>[2x]MTTFLIKHKASGKFLHPYGGSSNPANNTKLVLHSDIHERMYFQFDVVDERWGYIKHVASGKIVHP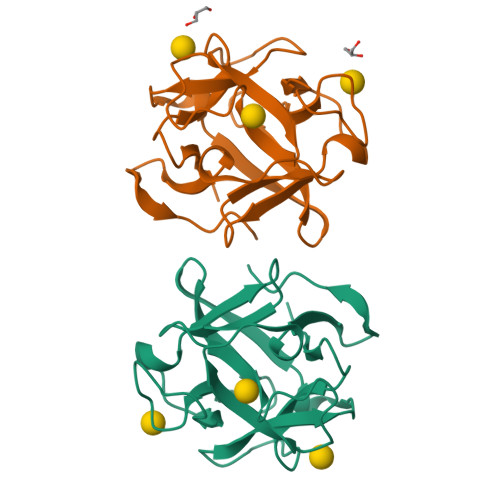YGGQANPPNETNMVLHQDRHDRALFAMDFFNDNIMHKGGKYIHPKGGSPNPPNNTETVIHGDKHAAMEFIFVSPKNKDKRVLVYAHHHHHH>[2x]MRFIHALLLAGIAHSAYASEKLTFKTDLEKLEREKAAQIGVAIVDPQGEIVAGHRMAQRFAMCSTFKFPLAALVFERIDSGTERGDRKLSYGPDMIVEWSPATERFLASGHMTVLEAAQAAVQLSDNGATNLLLREIGGPAAMTQYFRKIGDSVSRLDRKEPEMSDNTPGDLRDTTTPIAMARTVAKVLYGGALTSTSTHTIERWLIGNQTGDATLRAGFPKDWVVGEKTGTCANGGR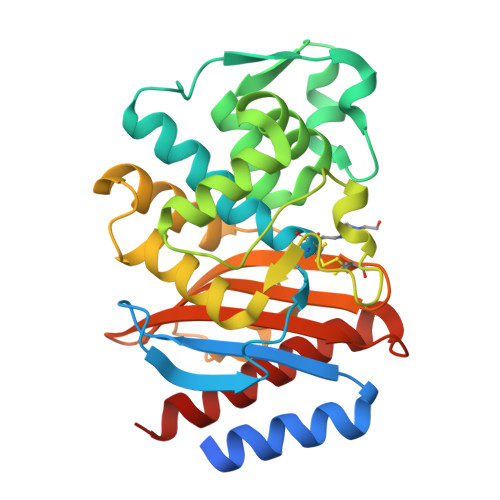NDIGFFKAQERDYAVAVYTTAPKLSAVERDELVASVGQVITQLILSTDK> MSSSSSTGYSKNNAAHIKQENTLRQRESSSISVSEELSSADERDAEDFSKEKPAAQSSLLRLESVVMPVIFTALALFTRMYKIGINNHVVWDEAHFGKFGSYYLRHEFYHDVHPPLGKMLVGLSGYLAGYNGSWDFPSGEIYPDYLDYVKMRLFNASFSALCVPLAYFTAKAIGFSLPTVWLMTVLVLFENSYSTLGRFILLDSMLLFFTVASFFSFVMFHNQRSKPF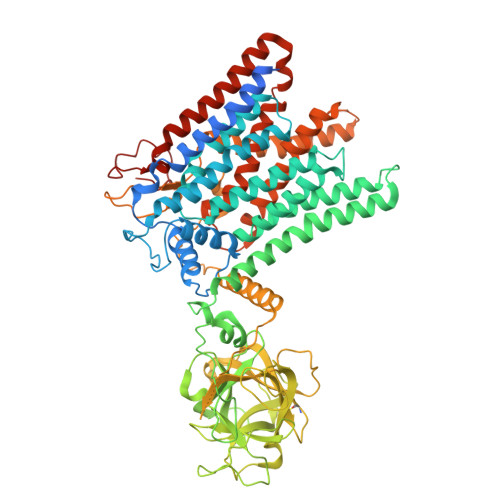SRKWWKWLLITGISLGCTISVKMVGLFIITMVGIYTVIDLWTFLADKSMSWKTYINHWLARIFGLIIVPFCIFLLCFKIHFDLLSHSGTGDANMPSLFQARLVGSDVGQGPRDIALGSSVVSIKNQALGGSLLHSHIQTYPDGSNQQQVTCYGYKDANNEWFFNRERGLPSWSENETDIEYLKPGTSYRLVHKSTGRNLHTHPVAAPVSKTQWEVSGYGDNVVGDNKDNWVIEIMDQRGDEDPEKLHTLTTSFRIKNLEMGCYLAQTGNSLPEWGFRQQEVVCMKNPFKRDKRTWWNIETHENERLPPRPEDFQYPKTNFLKDFIHLNLAMMATNNALVPDPDKFDYLASSAWQWPTLNVGLRLCGWGDDNPKYFLLGTPASTWASSVAVLAFMATVVILLIRWQRQYVDLRNPSNWNVFLMGGFYPLLAWGLHYMPFVIMSRVTYVHHYLPALYFALIILAYCFDAGLQKWSRSKCGRIMRFVLYAGFMALVIGCFWYFSPISFGMEGPSSNFRYLNWFSTWDIADKQEA> MKVQYCDSLVIGGGLAGLRAAVATQQKGLSTIVLSLIPVKRSHSAAAQGGMQASLGNSKMSDGDNEDLHFMDTVKGSDWGCDQKVARMFVNTAPKAIRELAAWGVPWTRIHKGDRMAIINAQKTTITEEDFRHGLIHSRDFGGTKKWRTCYTADATGHTMLFAVANECLKLGVSIQDRKEAIALIHQDGKCYGAVVRDLVTGDIIAYVAKGTLIATGGYGRIYKNTTNAVVCEGTGTAIALETGIAQLGNMEAVQFHPTPLFPSGILLTEGCRGDGGILRDVDGHRFMPDYEPEKKELASRDVVSRRMIEHIRKGKGVQSPYGQHLWLDISILGRKHIETNLRDVQEICEYFAGID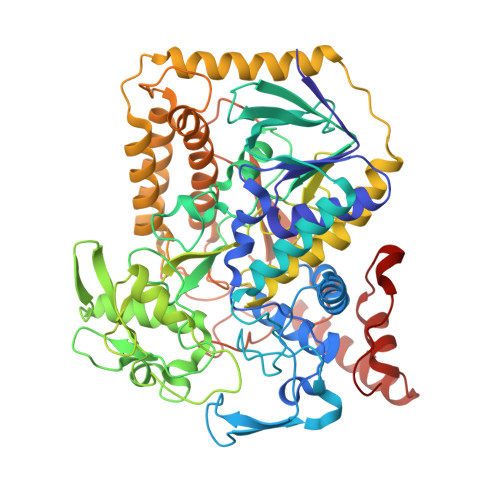PAEKWAPVLPMQHYSMGGIRTDYRGEAKLKGLFSAGEAACWDMHGFNRLGGNSVSEAVVAGMIVGEYFAEHCANTQVDLETKTLEKFVKGQEAYMKSLVESKGTEDVFKIKNRMKDVMDDNVGIFRDGPHLEKSVKELEELYKKSKNVGIKNKRLHANPELEEAYRVPMMLKVALCVAKGALDRTESRGAHNREDYPKRDDINWLNRTLASWPNPEQTLPTLEYEALDVNEMEIAPRYRGYGAKGNYIENPLSVKRQEEIDKIQSELEAAGKDRHAIQEALMPYELPAKYKARNERLGDK> 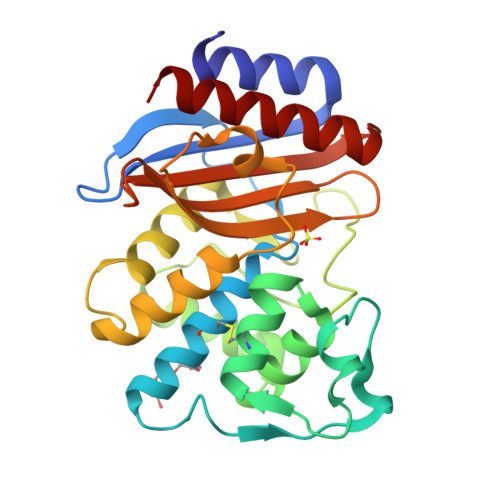HPETLVKVKDAEDQLGGRVGYIELDLASGKILESFRPEERFPMMSTFKVLLCGAVLSRVDAGQEQLGRRIHYSQNDLVEYSPVTEKHLTDGMTVGELCSAAITMSDNTAANLLLTTIGGPKELTAFLHNMGDHVTRLDRWEPELNEAIPNDERDTTTPVAMATTLRKLLTGELLTAASRQQLIDWMEADKVAGPLLRSALPAGWFIADKSGASERGSRGIIAALGPDGKPSRIVVIYMTGSQATMDERNRQIAEIGASLIKHW> HMSLSVANSTYETTALNSQKSSTDQPNSGSKSGQTLDLVNLGVAANFAILSKTGITDVYKSAITGDVGASPITGAAILLKCDEVTGTIFSVDAAGPACKITDASRLTTAVGDMQIAYDNAAGRLNPDFLNLGAGTIGGKTLTPGLYKWTSTLNIPTDITISGSSTDVWIFQVAGNLNMSSAVRITLAGGAQAKNIFWQTAGAVTLGSTSHFEGNILSQTGINCKTAASINGRMMAQTAVTLQMCTVTIPQ

The FfIBP from Flavobacterium frigoris PS1 exhibits high TH activity and relatively strong recrystallization inhibition activity. The FfIBP structure is composed of parallel β-strands in a helical pattern, which is mainly stabilized by inner hydrophobic interactions and intramolecular hydrogen bonds with long α415. Additionally, the FfIBP has a capping head region that consists of two small turns and β-strands, which contain a disulfide bond. This disulfide bond increases the overall rigidity of the protein and reduces residual movement at the ice-binding site, thereby augmenting TH activity and protein stability.

Based on the CD and MD simulation data, four mutants annotated as FfIBP_CC1 (A101C-A120C), FfIBP_CC2 (S96C-L132C), FfIBP_CC3 (M249C-N270C), and FfIBP_CC4 (G160C-S176C), possibly forming disulfide bonds, were generated. The formation of the disulfide bond at FfIBP_CC3 is anticipated to increase the stability of the global structure as the hyperactive IBPs contain disulfide bond(s) for the intra-interaction inside of the body domain. Therefore, we generated the FfIBP_CC3, which was located in the internal body domain. To confirm the disulfide formation, we solved the crystal structures of the FfIBP_CC1, CC2, CC3, and CC4 at 2.0, 2.1, 2.0, and 2.0 Å, respectively. Successful formation of the disulfide bond at the intended location in FfIBP_CC1 and FfIBP_CC4 was confirmed by X-ray crystallography, whereas the rest did not form a disulfide bond. The failure to form a disulfide bond may be due to dihedral angle constraints and the inappropriate distance between the two cysteines. When the RMSD values of alpha carbon mutants were compared with the wildtype, relatively high RMSD values exceeding 0.4 Å were observed around the mutation sites of FfIBP_CC2, FfIBP_CC3, and FfIBP_CC4. FfIBP_CC3 exhibited a ΔTm of − 0.8 °C compared to the wildtype, which is consistent with the hypothesis that the body region is heat-insensitive.>[30x]MTTKKFDEADKSNVEMYLIQAGVKQDAAATMGIWTAQELHRIKSQSYEEDYPVGSALRVFPVTTELSPTDKTFEYMTFDKVGTAQIIADYTDDLPLVDALGTSEFGKVFRLGNAYLISIDEIKAGQATGRPLSTRKASACQLAHDQLVNRLVFKGSAPHKIVSVFNHPNITKITSGKWIDASTMKPETAEAELTQAIETIETITRGQHRATNILIPPSMRKVLAIRMPETTMSYLDYFKSQNSGIEIDSIAELEDIDGAGTKGVLVYEKNPMNMSIEIPEAFNMLPAQPKDLHFKVPCTSKCTGLTIYRPMTIVLITGV;>MAQINASYQRDMAIALPGMVADTSKYNIDGACVVNEGDVLVGAAVQVVQAQAVDGHKLVKALTTGTTPYGVAIRSHWQTVNAQNQMIYEDGGAINVMTSGRVWMLSKSTEAPTFGSAVKLDVDGQEKSDGTIETTWTYAGGWTKYKDIQLVEVQLHQL[30x];>MAYENLFLRPACPGNISDTSTYNIDGACVAQGDIGFGSAVQVVGIVDGVKVVAALPDGGTPYGIAFRSQYEHLSGKILDGEVCNVVSHGRVWTLTSLGEAPSLFSKLQFGSGGVVTGGSGSAGWTFAGGFVKHEDGYIIEVQVKQNAFIAPPPPPPVVLVESATIATDKESPQPNNVTIQCVANALPDNATDKTGKWSIDATNIATVDPDSGLVTPVGGEVVGDFNITWTANDASKTTATIAYRVEAVPTPEVDA[5x];>MRYNQGCQLTAF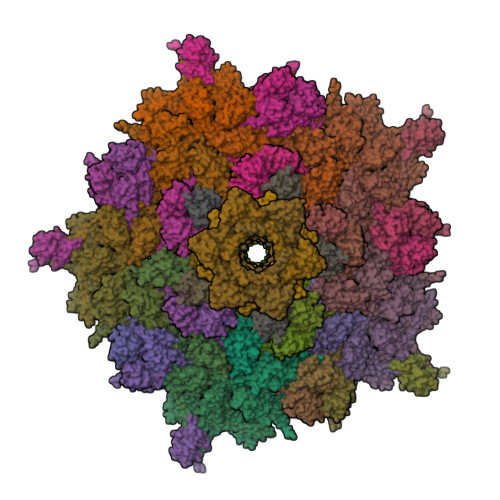FIGGNMKIVKHDGYNDIFNGGADGSPKPFFMSDASYHVGSFYNDNATAKRIVDVIPEEMVTAGFKISGVKDEKEFKSLWDSYKIDPSLVDALCWARLYGGAAIVAIINDNRMLTSPVKPGAKLEGVRVYDRFAITIEKRVTNARSPRYGEPEIYKVSPGDNIQPYLIHHTRIFIADGERVTPQMRKQNQGWGASVLNKSLIDAICDYDYCESLATQILRRKQQAVWKVKGLAEMCDDDDAQYAARLRLAQVDDNSGVGRAIGIDAETEEYDVLNSDISGVPEFLSSKMDRIVSLSGIHEIIIKNKNVGGVSASQNTALETFYKLVDRKREEDYRPLLEFLLPFIVDEQEWSIEFEPLSVPSKKEESEITKNNVESVTKAITEQIIDLEEARDTLRSIAPEFKLKDGNNINIREPEEPTEPEPGLGEKLEDEN[12x];>[6x]MHYELSAAARAAFLSKYRDFPHYMENRNFTPPKDGGMWLRFNYIEGDTLYLSIDRKCKSYIAIVQIGVVFPPGSGVDEARLKAKEIADFFKDGKMLNVGYIFEGAIVHQIVKHESGWMIPVRFTVRVDTKET;>[12x]MGVIMNQETLIAAVEQMRKLVPALRKVPDETLYAWVEMAELFVCQKTFKDAYVKAIALYALHLAFLDGALKGEDEDLESYSRRVTSFSLSGEFSQTFGEVTKNQSGNMMLSTPWGKMFEQLKARRRGRFALMTGLRGGCH;>MHLPNGAQIFVETSRGEEIEATAVTNEKNPVATVASKGDLAKGDYVIVTQSTWAKMVSRVLIVTDAQETSITLAGIDTSDTLVFPAGGTMSFAKITGWTEIPCVQEIGQDGGEQQYYTYQCLSDDKEQQIPTFKSAISLTYTFAHEFDNPIYQILRKLDSSGQVTAVRMYVPKASEMRMWAGILSFNDIPSTQVNEMETVELAVSLKGDFTFISSTLASPGA[6x];>[6x]MNYSQIERMARKGVAFFTDPSRPMNLIKQGEYGYDENGFEIPPMEQVIPISGATRRPNAREIDGETIRASDILGIFNNDHEINEGDYIEIDGIRHVVVDARPVQASLEPVAYRPVLRRVSVGG> MAHHHHHHSSGLEVLFQGPDLHVIDHDFLKGQGDARSVRHIAIPAHRGLITDRNGEPLAVSTPVTTLWANPKELMTAKERWPQLAAALGQDTKLFADRIEQNAEREFIYLVRGLTPEQGEGVIALKVPGVYSIEEFRRFYPAGEVVAHAVGFTDVDDRGREGIELAFDEWLAGVPGKRQVLKDRRGRVIKDVQVTKNAKPGKTLALSIDLRLQYLAHRELRNALLENGAKAGSLVIMDVKTGEILAMTNQPTYNPNNRRNLQPAAMRNRAMIDVFEPGSTVKPFSMSAALASGRWKPSDIVDVYPGTLQIGRYTIRDVSRNSRQLDLTGILIKSSNVGISKIAFDIGAESIYSVMQQVGLGQDTGLGFPGERVGNLPNHRKWPKAETATLAYGYGLSVTAIQLAHAYAALANDGKSVPLSMTRVDRVPDGVQVISPEVASTVQGMLQQVVEAQGGVFRAQVPGYHAAGKSGTARKVSVGTKGYRENAYRSLFAGFAPATDPRIAMVVVIDEPSKAGYFGGLVSAPVFSKVMAGALRLMNVPPDNLPTATEQQQVNAA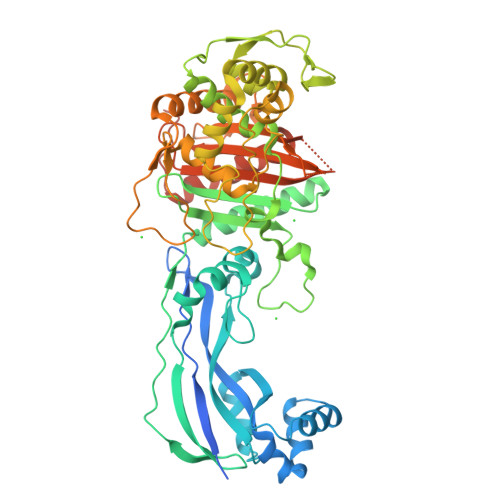PAKGGRG The autonomous non-LTR retrotransposon long interspersed nuclear element-1 (LINE-1 or L1) is one the most abundant mobile elements in the human genome, comprising 17–20% of its content. ORF1p acts as a nucleic acid chaperone that binds L1 RNA, while ORF2p provides endonuclease (EN), reverse transcriptase (RT) and RNA-binding activities through three distinct functional domains. L1-EN initiates de novo L1 integration by producing a single-strand nick at a genomic site generally fitting the consensus target sequence 5′-TTTTT/AA-3′ (6,7,24,25). L1-EN belongs to the family of metal-dependent phosphohydrolases that includes apurinic/apyrimidinic endonuclease 1 (APE1) and DNase I, which are part of the exonuclease-endonuclease-phosphatase (EEP) domain superfamily.

To confirm the position of the catalytic metal in L1-EN, we soaked crystals of WT L1-EN (formed without DNA) with 20 mM MgCl2 during cryoprotection and refined the structure to 2.0 Å resolution. We modeled a Mg-water cluster with four water molecules at the electron density near Glu43. In addition to the four water molecules coordinated by Mg2+, there were other water molecules near the active site. The one with the strongest electron density is coordinated by Asp145 (2.6 Å) and Asn147 (2.7 Å). Notably, Asp145 and corresponding aspartic acids in DNase I and APE1 were proposed to activate nucleophilic water during catalysis. Upon superposition of our Mg-bound L1-EN structure with the structures of our DNA-bound L1-EN complexes, distances between the modeled Mg2+ and the scissile bond OP2 are 3.8 Å for B-form DNA and 1.4 Å for the alternative conformation with the phosphate rotated. We modeled a L1-EN-DNA complex with a bound Mg2+ ion by forcefield relaxation in the mixed constraints with active site amino acids around Mg2+ coming from our structure of Mg2+-bound WT L1-EN without DNA and the rest of the amino acids coming from our structure of L1-EN-D145A/Y226K complexed with dna14. Indeed, when modeled into the rotated phosphate DNA conformation, the transient holo-phosphate moiety became strongly coordinated by the Mg2+ ion via two of its oxygen atoms (at 2.0 Å and 2.1 Å from Mg2+), replacing the two water molecules and maintaining near-octahedral Mg2+ coordination. Notably, about halfway through the rotation, the phosphate approaches W5, which is coordinated by Asp145 and favorably positioned for nucleophilic attack on the phosphate. Asp145 carboxylate may serve as a general base that accepts a proton from W5, thus liberating the hydroxyl anion. pKa estimation for Asp145 using PROPKA indicated a strong upshift of pKa = 6.5 for this side chain, in agreement with a general base function.

>[2x]MTGSNSHITILTLNINGLNSAIKRHRLASWIKSQDPSVCCIQETHLTCRDTHRLKIKGWRKIYQANGKQKKAGVAILVSDKTDFKPTKIKRDKEGHYIMVKGSIQQEELTILNIYAPNTGAPRFIKQVLSDLQRDLDSHTLIMGDFNTPLSTLDRSTRQKVNKDTQELNSALHQADLIDIYRTLHPKSTEYTFFSAPHHTYSKIDHIVGSKALLSKCKRTEIITNYLSDHSAIKLELR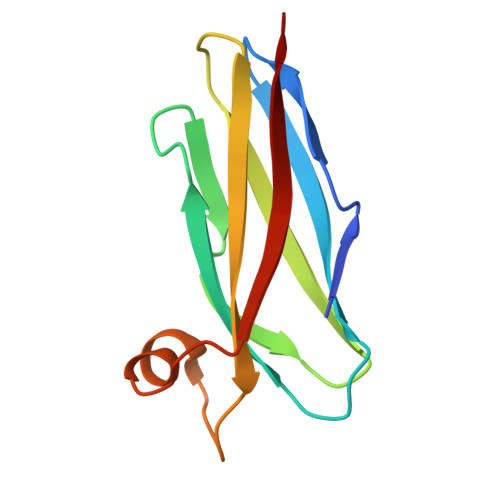>[2x]MSLTADPPACTVPAAGVSSTHKLVNGGAEKIVFKIKSSNNNEYRIAPVFGFVDPSGSKDVVITRTAGAPKEDKLVVHFASAPADATDAQAAFVAVAPAGTVTIPMSATA Gram-negative species couple polymerization with translocation across the periplasm and outer membrane and the master regulator of the system is the tyrosine autokinase, Wzc. The tyrosine autokinase domain forms the cytoplasm region, while the periplasmic region contains small folded motifs and helical bundles. Autophosphorylation of the tyrosine-rich C-terminus of Wzc results in disassembly of the octamer into multiply phosphorylated monomers. We propose that the cycling between phosphorylated monomer and dephosphorylated octamer regulates glycan polymerization and translocation.

Reasoning the negatively charged Glu would mimic negatively charged pTyr (phosphotyrosine) and create a protein resembling a locked phosphorylated state, several Tyr-to-Glu mutants were constructed in WzcK540M. Analysis of cryo-EM images of WzcK540M with four Glu residues (designated WzcK540M4YE) revealed ~50% octamers, as well as other state(s). A 2.8 Å-resolution structure of the WzcK540M4YE octamer was determined using the same approach as WzcK540M. Overall, this structure has similar octameric (rmsd 3.1 Å over 4520 Cα atoms) and monomeric (rmsd of 2.5 Å over 651 Cα atoms) arrangements seen in WzcK540M. The core kinase domain is unchanged between the structures (rmsd 0.4 Å for Cα atoms 452–697) but the tyrosine-rich tail has undergone a large change that now places Y708 at the active site (compared Y717 in WzcK540M). Motif 3 still possesses the same three structural arrangements seen in WzcK540M but only two (not three) monomers have the fully ordered class i arrangement (rmsd of 0.4 Å for 133 Cα atoms). The larger rmsd value for the monomer and octamer, compare to the individual regions, reflects shifts in the relative positions of the regions. This can be visualised by superimposing the core kinase domains of monomer for WzcK540M and WzcK540M4YE, which shows a rigid body rotation of 11° at the other end of the molecule. Superposition using all the Cα atoms in octamer reveals shifts in the periplasmic helices, particularly those in class ii. Comparing WzcK540M vs WzcK540M4YE revealed the distribution of arrangements changed, suggesting the helical bundles are particularly sensitive to changes elsewhere in the structure. The structure of WzcK540M4YE, chosen to mimic a phosphorylated state, showed a significant conformational change in the tyrosine tail, which would be predicted to weaken the octamer.

>[8x]MTSVTSKQSTILGSDEIDLGRVIGELIDHRKLIISITSVFTLFAILYALLATPIYETDALIQIEQKQGNAILSSLSQVLPDGQPQSAPETALLQSRMILGKTIDDLNLQIQIEQKYFPVIGRGLARLMGEKPGNIDITRLYLPDSDDISNNTPSIILTVKDKENYSINSDGIQLNGVVGTLLNEKGISLLVNEIDAKPGDQFVITQLPRLKAISDLLKSFSVADLGKDTGMLTLTLTGDNPKRISHILDSISQNYLAQNIARQAAQDAKSLEFLNQQLPKVRAELDSAEDKLNAYRKQKDSVDLNMEAKSVLDQIVNVDNQLNELTFREAEVSQLYTKEHPTYKALMEKRQTLQEEKSKLNKRVSSMPSTQQEVLRLSRDVESGRAVYLQLLNRQQELNIAKSSAIGNVRIIDNAVTDPNPVRPKKTIIIVIGVVLGLIVSVVLVLFQVFLRRGIESPEQLEEIGINVYASIPISEWLTKNARQSGKVRKNQSDTLLAVGNPADLAVEAIRGLRTSLHFAMMEAKNNVLMISGASPSAGMTFISSNLAATIAITGKKVLFIDADLRKGYAHKMFGHKNDKGLSEFLSGQAAAEMIIDKVEGGGFDYIGRGQIPPNPAELLMHPRFEQLLNWASQNYDLIIIDTPPILAVTDAAIIGRYAGTCLLVARFEKNTVKEIDVSMKRFEQSGVVVKGCILNGVVKKASSYYRYGHNHEGESEEDKKHHHHHH> MAPKKQEQEPIRLSTRTASKKVDYLQLSNGKLEDFFDDLEEDNKPARNRSRSKKRGRKPLKKADSRSKTPSRVSNARGRSKSLGPRKTYPRKKNLSPDNQLSLLLKWRNDKIPLKSASETDNKCKVVNVKNIFKSDLSKYGANLQALFINALWKVKSRKEKEGLNINDLSNLKIPLSLMKNGILFIWSEKEILGQIVEIMEQKGFTYIENFSIMFLGLNKCLQSINHKDEDSQNSTASTNNTNNEAITSDLTLKDTSKFSDQIQDNHSEDSDQARKQQTPDDITQKKNKLLKKSSVPSIQKLFEEDPVQTPSVNKPIEKSIEQVTQEKKFVMNNLDILKSTDINNLFLRNNYPYFKKTRHTLLMFRRIGDKNQKLELRHQRTSDVVFEVTDEQDPSKVDTMMKEYVYQMIETLLPKAQFIPGVDKHLKMMELFASTDNYRPGWISVIEK;> MSKAVNKKGLRPRKSDSILDHIKNKLDQEFLEDNENGEQSDEDYDQKSLNKAKKPYKKRQTQNGSELVISQQKTKAKASANNKKSAKNSQKLDEEEKIVEEEDLSPQKNGAVSEDDQQQEASTQEDDYLDRLPKSKKGLQGLLQDIEKRILHYKQLFFKEQNEIANGKRSMVPDNSIPICSDVTKLNFQALIDAQMRHAGKMFDVIMMDPPWQLSSSQPSRGVAIAYDSLSDEKIQNMPIQSLQQDGFIFVWAINAKYRVTIKMIENWGYKLVDEITWVKKTVNGKIAKGHGFYLQHAKESCLIGVKGDVDNGRFKKNIASDVIFSERRGQSQKPEEIYQYINQLCPNGNYLEIFARRNNLHDNWVSIGNEL;> MSLKKGKFQHNQSKSLWNYTLSPGWREEEVKILKSALQLFGIGKWKKIMESGCLPGKSIGQIYMQTQRLLGQQSLGDFMGLQIDLEAVFNQNMKKQDVLRKNNCIINTGDNPTKEERKRRIEQNRKIYGLSAKQIAEIKLPKVKKHAPQYMTLEDIENEKFTNLEILTHLYNLKAEIVRRLAEQGETIAQPSIIKSLNNLNHNLEQNQNSNSSTETKVTLEQSGKKKYKVLAIEETELQNGPIATNSQKKSINGKRKNNRKINSDSEGNEEDISLEDIDSQESEINSEEIVEDDEEDEQIEEPSKIKKRKKNPEQESEEDDIEEDQEEDELVVNEEEIFEDDDDDEDNQDSSEDDDDDED;> MKHHHHHHHGAAGTSLYKKAGENLYFQGSMKKNGKSQNQPLDFTQYAKNMRKDLSNQDICLEDGALNHSYFLTKKGQYWTPLNQKALQRGIELFGVGNWKEINYDEFSGKANIVELELRTCMILGINDITEYYGKKISEEEQEEIKKSNIAKGKKENKLKDNIYQKLQQMQ

The Tetrahymena thermophila MTA1 complex consisting of four subunits, namely MTA1, MTA9, p1, and p2, is the first identified eukaryotic 6mA methyltransferase (MTase) complex. The MTA1 complex comprises four protein subunits, namely MTA1, MTA9, p1, and p230. Both MTA1 and MTA9 contain the MT-A70 domain that is widely involved in eukaryotic RNA m6A modification, but only MTA1 contains the conserved catalytic DPPW motif, which is reminiscent of the heterodimeric RNA m6A MTase subunits METTL3 and METTL1433–35. Neither MTA1 nor MTA9 has a nucleic acid binding domain, and p1 and p2, two homeobox-like DNA-binding proteins, are required for the MTA1 complex’s MTase activity. Coupled with biochemical characterization, we revealed that MTA1 serves as the catalytic core, MTA1, MTA9, and p1 likely accommodate the substrate DNA, and p2 may facilitate the stabilization of MTA1.

After extensive cryo-EM screening (detailed in Materials and methods), we obtained SAM- and SAH-bound MTA1 complexes and determined their structures at average resolutions of 2.6 Å and 2.8 Å, respectively. As the two structures are almost identical, for simplicity we focused on the higher-resolution SAM-bound MTA1 complex and described the structures of the components in detail. The SAM-bound MTA1 complex overall exhibits an “L” shape architecture, with MTA1–MTA9 and p1–p2 perpendicular to each other. Specifically, MTA1 shows extensive contacts with MTA9 on one side, while on the other side the MTA1 N-terminal helix (NH) protrudes from the direction perpendicular to the surfaces of MTA1 and MTA9 and directly interacts with p1 and p2. The co-factor substrate SAM is found in the MTase domain of MTA1. Specifically, the SAM molecule is positioned at the end of MTA1 β2, β7, and β8, facing the conserved DPPW catalytic motif (residues 209–212) in MTA1. The adenine moiety of SAM is recognized by the side chain of D182 and the main chain of V183 in MTA1. The hydroxyl groups of ribose are surrounded by MTA1 N370, E371, and R357. Several residues, including D209, S332, and N360, directly contact the methionine moiety of SAM. In MTA9, SAM is not found and an eroded NALW motif is observed instead of the conventional catalytic DPPW motif.> MELTPREKDKLLLFTAALVAERRLARGLKLNYPESVALISAFIMEGARDGKSVASLMEEGRHVLTREQVMEGVPEMIPDIQVEATFPDGSKLVTVHNPII;> MIPGEYHVKPGQIALNTGRATCRVVVENHGDRPIQVGSHYHFAEVNPALKFDRQQAAGYRLNIPAGTAVRFEPGQKREVELVAFAGHRAVFGFRGEVMGPLEVNDE;> MSNISRQAYADMFGPTVGDKVRLADTELWIEVEDDLTTYGEEVKFGGGKVIRDGMGQGQMLAADCVDLVLTNALIVDHWGIVKADIGVKDGRIFAIGKAGNPDIQPNVTIPIGAATEVIAAEGKIVTAGGIDTAIHWICPQQAEEALVSGVTTMVGGGTGPAAGTHATTCTPGPWYISRMLQAADSLPVNIGLLGKGNVSQPDALREQVAAGVIGLKIHEDWGATPAAIDCALTVADEMDIQVALHSDTLNESGFVEDTLAAIGGRTIHTFHTEGAGGGHAPDIITACAHPNILPSSTNPTLPYTLNTIDEHLDMLMVCHHLDPDIAEDVAFAESRIRRETIAAEDVLHDLGAFSLTSSDSQAMGRVGEVILRTWQVAHRMKVQRGALAEETGDNDNFRVKRYIAKYTINPALTHGIAHEVGSIEVGKLADLVVWSPAFFGVKPATVIKGGMIAIAPMGDINASIPTPQPVHYRPMFGALGSARHHCRLTFLSQAAAANGVAERLNLRSAIAVVK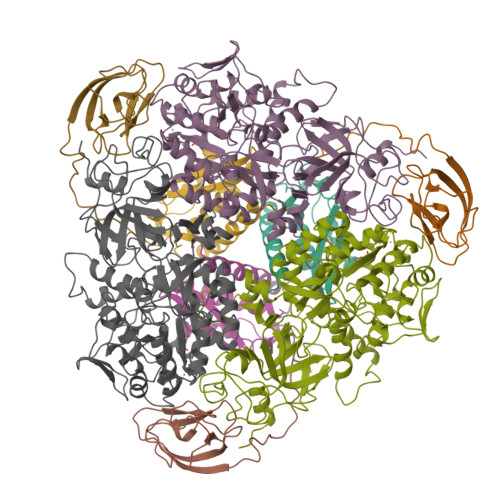GCRTVQKADMVHNSLQPNITVDAQTYEVRVDGELITSEPADVLPMAQRYFLF> GPHMLD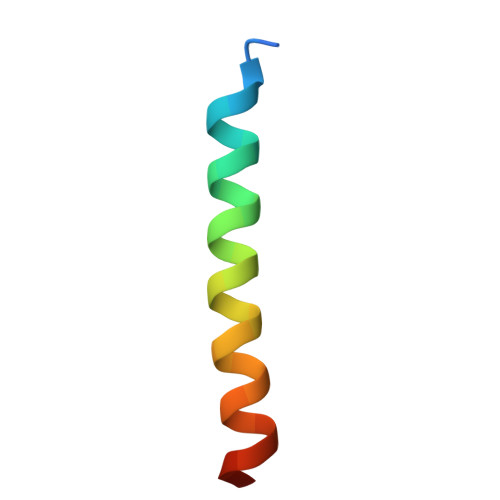NFMKQLLKLEESLNKLELEQKVTNKE> QGPLGSSKVSEQLKCCSGILKEMFAKK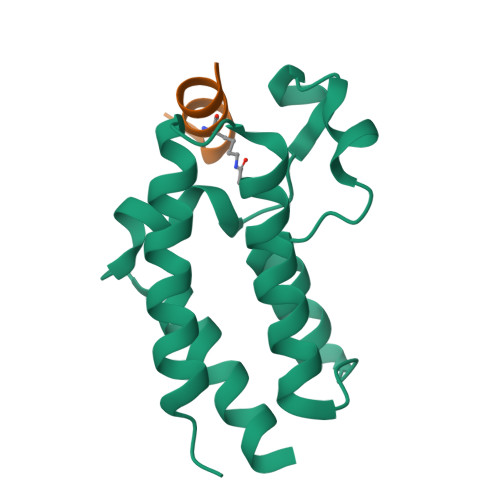HAAYAWPFYKPVDVEALGLHDYCDIIKHPMDMSTIKSKLEAREYRDAQEFGADVRLMFSNCYKYNPPDHEVVAMARKLQDVFEMRFAKMPDEPEEP;> XWSWLCKKYNLIH> SQPNATLYKMSSINADFAFNLYRRFTVETPDKNIFFSPVSISAALVMLSFGACCSTQTEIVETLGFNLTDTPMVEIQHGFQHLICSLNFPKKELELQIGNALFIGKHLKPLAKFLNDVKTLYETEVFSTDFSNISAAKQEINSHVEMQTKG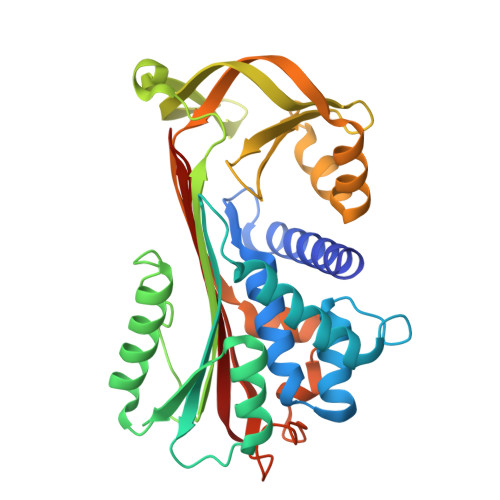KVVGLIQDLKPNTIMVLVNYIHFKAQWANPFDPSKTEDSSSFLIDKTTTVQVPMMHQMEQYYHLVDMELNCTVLQMDYSKNALALFVLPKEGQMESVEAAMSSKTLKKWNRLLQKGWVDLFVPKFSISATYDLGATLLKMGIQHAYSENADFSGLTEDNGLKLSNAAHKAVLHIGEKGTEAAGAMFLEAIPR> MSPFPLTSMDKAFITVLEMTPVLGTEIINYRDGMGRVLAQDVYAKDNLPPFPASVKDGYAVRAADGPGDRFIIGESQAGEQPTQTVMPGQVMRVTTGAPIPCGADAVVQVEDTELIRESDDGTEELEVRILVQARPGQDIRPIGHDIKRGECVLAKGTHMGPSEIGLLATVGVTEVEVNKFPVVAVMSTGNELLNPEDDLLPGKIRDSNRSTLLATIQEHGYPTINLGIVGDNPDDLLNALNEGISRADVIITSGGVSMGEKDYLKQVLDIDLHAQIHFGRVFMKPGLPTTFATLDIDGVRKIIFALPGNPVSAVVTCNLFVVPALRKMQGILDPRPTIIKARLSCDVKLDPRPEYHRCILTWHHQ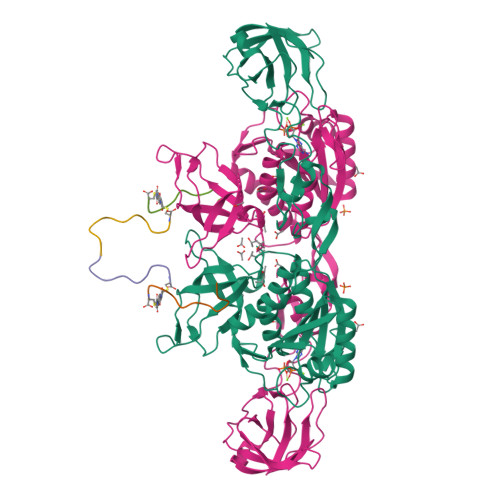EPLPWAQSTGNQMSSRLMSMRSANGLLMLPPKTEQYVELHKGEVVDVMVIGRL;>FSIVGSLPRDC[2x]N-benzyl-1-{5-[(2-chloro-5-{5-(methylsulfonyl)-1-[3-(morpholin-4-yl)propyl]-4,5,6,7-tetrahydro-1H-pyrazolo[4,3-c]pyridin-3-yl}phenyl)ethynyl]-2-methoxyphenyl}methanamine 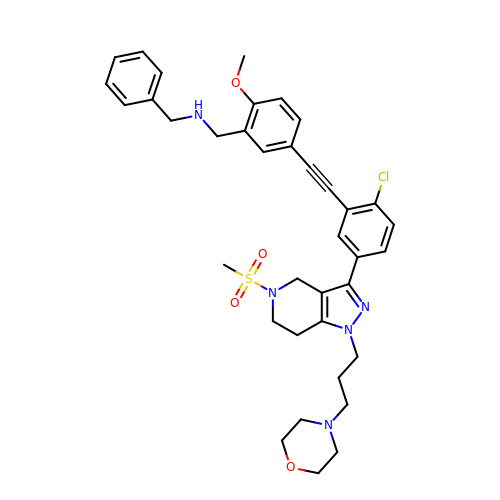| C37 H42 Cl N5 O4 S | XDJYRFZPTINNSF-UHFFFAOYSA-N> GSTVQVPYTITVNGTSQNILSNLTFN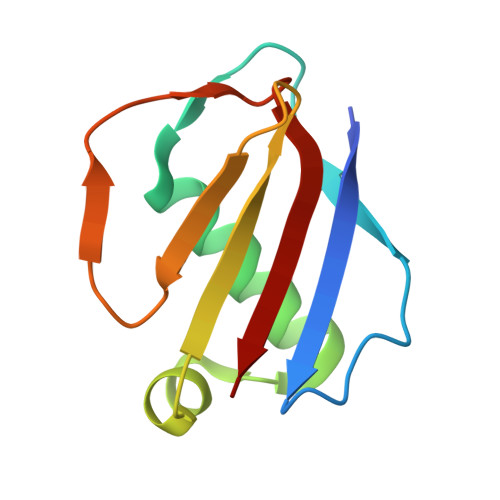KNQNISYKDLEGKVKSVLESNRGITDVDLRLSKQAKYTVNFKNGTKKVIDLKSGIYTANLINSSDIKSININVD> GSKWKVFIDQINRSLENYEPCSSQNCSCYHGVIEEDLTPFRGGISRKMMAEVVRRKLGTHYQITKNRLYRENDCMFPSRCSGVEHFILEVIGRLPDMEMVINVRDYPQVPKWMEPAIPVFSFSKTSEYHDIMYPAWTFWEGGPAVWPIYPTGLGRWDLFREDLVRSAAQWPWKKKNSTAYFRGSRTSPERD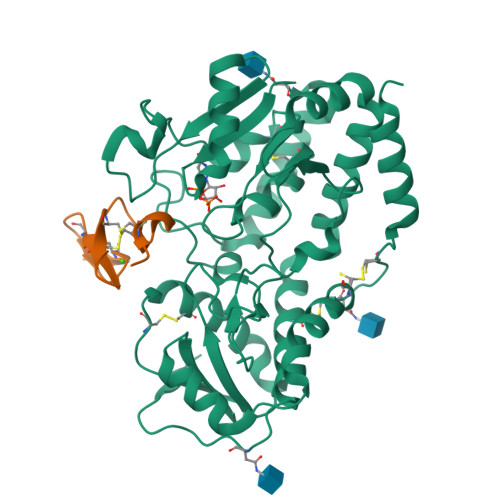PLILLSRKNPKLVDAEYTKNQAWKSMKDTLGKPAAKDVHLVDHCKYKYLFNFRGVAASFRFKHLFLCGSLVFHVGDEWLEFFYPQLKPWVHYIPVKTDLSNVQELLQFVKANDDVAQEIAERGSQFIRNHLQMDDITCYWENLLSEYSKFLSYNVTRRKGYDQIIP;> GSDVNECVTNPCQNDATCLDQIGEFQCICMPGYEGVHCEVNT> TLPKPFIWAEPHFMVPKEKQVTICCQGNYGAVEYQLHFEGSLFAVDRPKPPERINKVKFYIPDMNSRMAGQYSCIYRVGELWSEPSNLLDLVVTEMYDTPTLSVHPGPEVISGE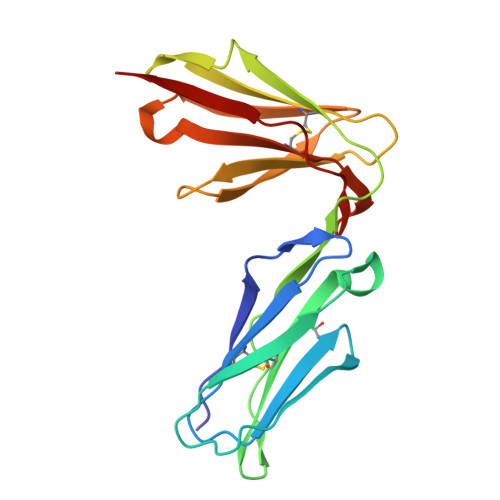KVTFYCRLDTATSMFLLLKEGRSSHVQRGYGKVQAEFPLGPVTTAHRGTYRCFGSYNNHAWSFPSEPVKLLVTG>SAFDQAARSRGHSNRRTALRPRRQQEATEVRPEQKMPTLLRVYIDGPHGMGKTTTTQLLVALGSRDDIVYVPEPMTYWRVLGASETIANIYTTQHRLDQGEISAGDAAVVMTSAQITMGMPYAVTDAVLAPHIGGEAGSSHAPPPALTLIFDRHPIAALLCYPAARYLMGSMTPQAVLAFVALIPPTLPGTNIVLGALPEDRHIDRLAKRQRPGERLDLAMLAAIRRVYGLLANTVRYLQCGGSWREDWGQLSGTAVPPQGAEPQSNAGPRPHIGDTLFTLFRAPELLAPNGDLYNVFAWALDVLAKRLRSMHVFILDYDQSPAGCRDALLQLTSGMVQTHVTTPGSIPTICDLARTFAREMG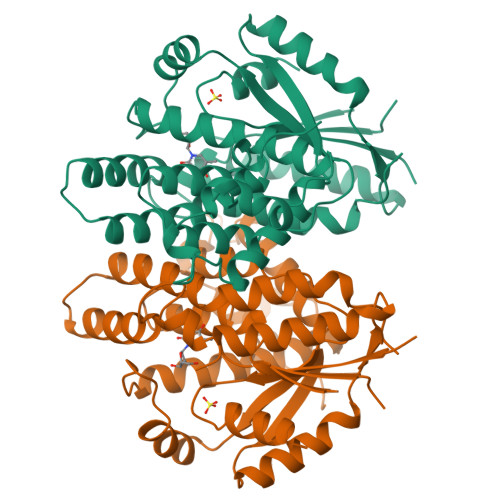EAN[2x]> SESSIENFLCRSACVYMGEYHTTNTDTSKLFASWTINARRMVQMRRKLELFTYVRFDMEVTFVITSKQDQGTQLGQDMPPLTHQIMYIPPGGPIPKSVTDYTWQTSTNPSIFWTEGNAPPRMSIPFISIGNAYSNFYDGWSHFSQNGVYGYNTLNHMGQIYV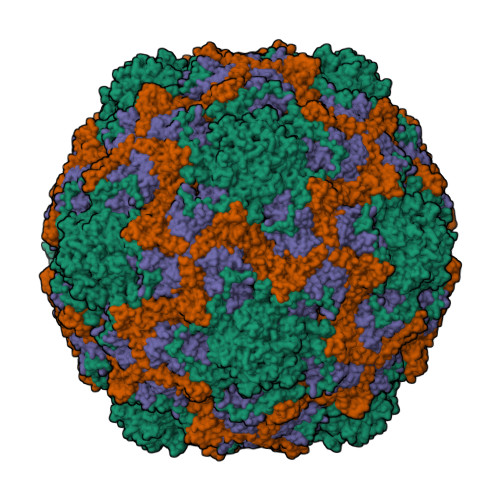RHVNGSSPLPMTSTVRMYFKPKHVKVWVPRPPRLCQYKNASTVNFTPTNITEKRQSINYIPETV;> RVRSITLGNSTITTQESANVVVAYGRWPEYLKDNEATAEDQPTQPDVATCRFYTLESVTWERDSPGWWWKFPDALKDMGLFGQNMYYHYLGRAGYTIHVQCNASKFHQGCLMVVCVPEAEMGCSQVDGTVNEHSLSEGETAKKFASTSTNGTNTVQSIVTNAGMGVGVGNLTIFPHQWINLRTNNCATIVMPYINNVPMDNMFRHHNFTLMIIPFVPLDYSSDSSTYVPITVTVAPMCAEYNGLR;> GLPVMNTPGSNQFLTSDDFQSPSAMPQFDVTPELNIPGEVQNLMEIAEVDSVVPVNNVEGKLDTMEIYRIPVQSGNHQSSQVFGFQVQPGLDNVFKHTLLGEILNYYAHWSGSIKLTFVFCGSAMATGKFLLAYAPPGANAPKSRKDAMLGTHIIWDVGLQSSCVLCIPWISQTHYRLVQQDEYTSAGNVTCWYQTGIVVPAGTPTSCSIMCFVSACNDFSVRLLKDTPFI> MGSHHHHHHSQDPNSMPARALLPRRMGHRTLASTPALWASIPCPRSELRLDLVLPSGQSFRWREQSPAHWSGVLADQVWTLTQTEEQLHCTVYRGDKSQASRPTPDELEAVRKYFQLDVTLAQLYHHWGSVDSHFQEVAQKFQGVRLLRQDPIECLFSFICSSNNNIARITGMVERLCQAFGPRLIQLDDVTYHGFPSLQALAGPEVEAHLRKLGLGYRARYVSASARAILEEQGGLAWLQQLRESSYEEAHKALCILPGVGTCVADKICLMALDKPQAVPVNVHMWHIAQRDYSWHPTTSQAKGPSPQTNKELGNFFRSLWGPYAGWAQAVLFSADLRQSRHAQEPPAKRRKGSKGP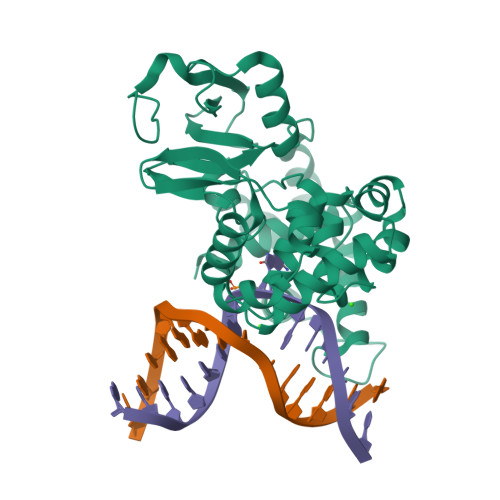EG> SLTRIDHIGIACHDLDATVEFYRATYGFEVFHTEVNEEQGVRLAMLKINDTSDGGASYL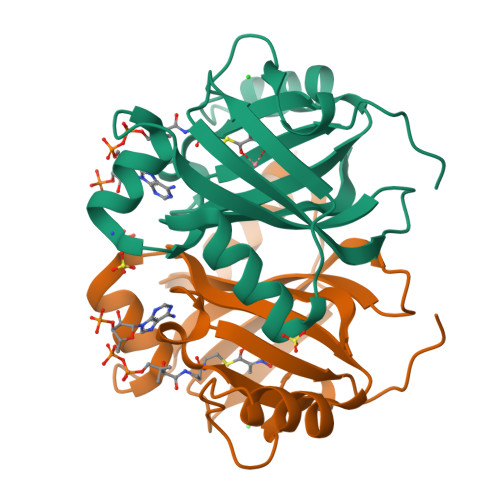QLLEPTREDSAVGKWLAKNGEGVHHIAFGTADVDADAADIRDKGVRVLYDEPRRGSMGSRITFLHPKDCHGVLTELVTSAAVESPEH RepB, the replication initiation protein of pMV158, is a member of the HUH endonuclease superfamily, which includes proteins involved in the replication of plasmids, bacteriophages and viruses, as well as proteins with roles in DNA transposition and in conjugative mobilisation of plasmids. These proteins are characterised by the presence of two conserved protein motifs: the HUH motif, composed of two His residues separated by a bulky hydrophobic amino acid, which is responsible for the coordination of a divalent metal cation, and the catalytic motif, containing one or two Tyr residues separated by several amino acids. Each monomer of RepB comprises two domains connected by a short hinge region. The C-terminal or oligomerisation domain (OD) is a helical domain responsible for the hexameric state of the protein, while the N-terminal or origin binding domain (OBD) carries the catalytic active site and is in charge of recognising, cleaving and joining dso DNA.

A very high-resolution 1.50 Å structure of the OBD alone was obtained. Although the crystals grew in the presence of ssDNA of the nick sequence, there was no DNA bound to the protein. The main differences observed are located on flexible regions, such as the loop between β-strands β2–β3, which includes the residues coordinating the Mn2+ metal ion (data not shown). However, alignment of these two structures reveals clear differences located in the flexible loop connecting β2 and β3 β-strands and in the loop connecting α2 and β4, due to its proximity to the DNA.

> MAKEKARYFTFLLYPESIPSDWELKLETLGVPMAISPLHDKDKSSIKGQKYKKAHYHVLYIAKNPVTADSVRKKIKLLLGEKSLAMVQVVLNVENMYLYLTHESKDAIAKKKHVYDKADIKLINNFDIDRYV2-O-phosphono-beta-L-arabinopyranose | C5 H11 O8 P | 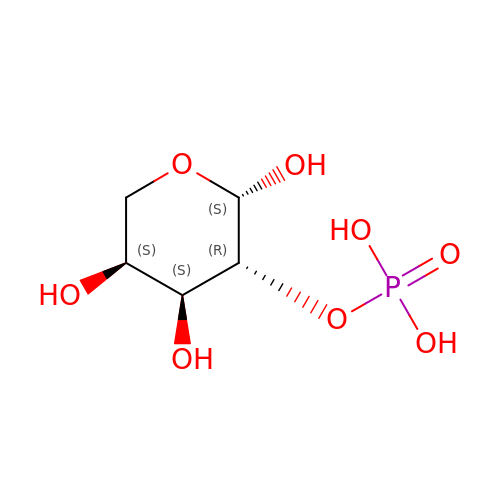QIAIUTJEZJIPSH-KLVWXMOXSA-N>[2x]ACYSELSVQHNLVVQGDFALTQTQMATYEHNFNDSSCVSTNTITPMSPSDIIVGLYNDTIKLNLHFEWTNKNNITLSN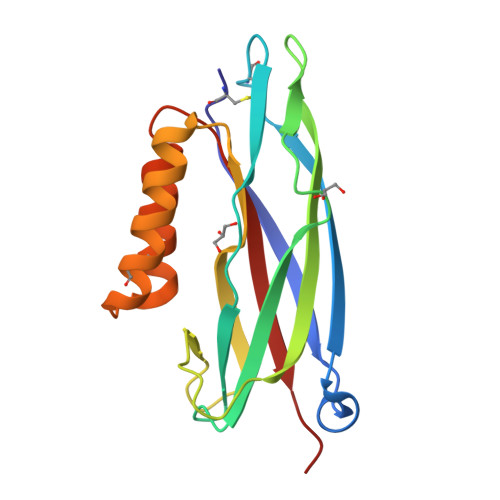NQTSFTSGYSVTVTPAASNAKVNVSAGGGGSVMINGVATLSSASSSTRGSAAVQFLLCLLGGKSWDACVNSARNALAQNAGVYSFNLTLSYNPIT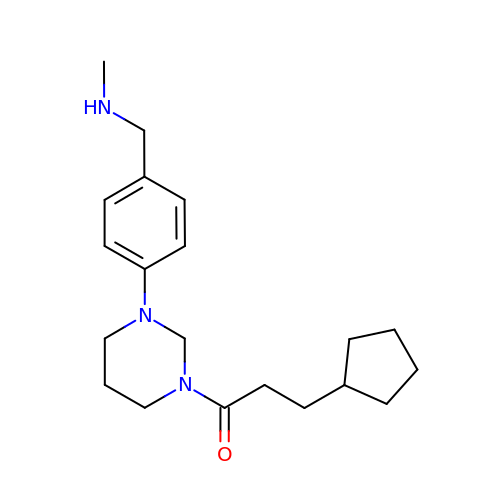3-cyclopentyl-1-[3-[4-(methylaminomethyl)phenyl]-1,3-diazinan-1-yl]propan-1-one | C20 H31 N3 O | FGLHMHLKBALILM-UHFFFAOYSA-N>[2x]MGSSHHHHHHSSENLYQFGHMMNKDSKIYIAGHTGLVGSSILKKLQNDGYENLIFRTHSELDLTNQQAVTDFFKKEKPEYVFFCAAKMGGMMEQLERRADFLYLNLIMQTFVLHEAYKNDCKKLLYL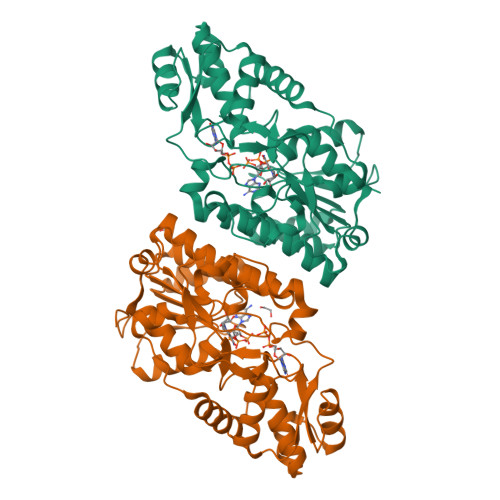SSLCIYPQDASLPIKETSMLEGKLQFINEPYAVAKITGNKMCEFYNQQFGTNFITLVPTSIYGPGDNFNLATAHVFPAIFAKIYLGKLLNEQKHQELFNSLRLDNIQDVLKYLSQFDIDENKVTLLGSGNPRREFIYVDDVADACIFTMDKIDASMLKKYDENFHNTHLNLADGKDYSIKEVAFLIKDIIGYKGDIIFDSSKLDGTMLKTTNTERIRKLGWKAKIKLEDGIKMMYEWYLKEQNIRQ> MGSSHHHHHHSSGLVPRASMLEAKFEEASLFKRIIDGFKDCVQLVNFQCKEDGIIAQAVDDSRVLLVSLEIGVEAFQEYRCDHPVTLGMDLTSLSKILRCGNNTDTLTLIADNTPDSIILLFEDTKKDRIAEYSLKLMDIDADFLKIEELQYDSTLSLPSSEFSKIVRDLSQLSDSINIMITKETIKFVADGDIGSGSVIIKPFVDMEHPETSIKLEMDQPVDLTFGAKYLLDIIKGSSLSDRVGIRLSSEAPALFQFDLKSGF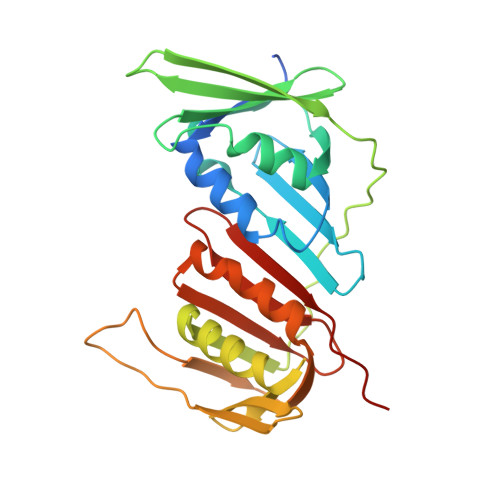LQFFLAPKFNDEE> IFLNVLEAIEPGVVCAGHDNNQPDSFAALLSSLNELGERQLVHVVKWAKALPGFRNLHVDDQMAVIQYSLMGLMVFAMGWRSFTNVNSRMLYFAPDLVFNEYRMHKSRMYSQCVRMRHLSQEFGWLQITPQEFLCMKALLLFSIIPVDGLKNQKFFDELRMNYIKELDRII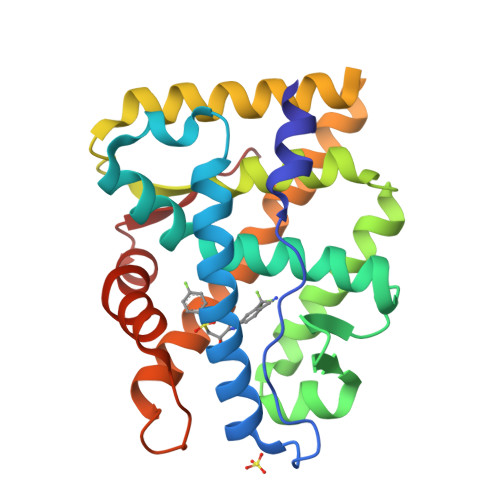ACKRKNPTSCSRRFYQLTKLLDSVQPIARELHQFTFDLLIKSHMVSVDFPEMMAEIISVQVPKILSGKVKPIYFH>[2x]GEFMEEGKMDENEWSYHGEGNKSLVVAHAQRCVVLRFLKFPPNKKKTSEEILQHLQNIVDFGKNVMKDFLGENYVHCGEVVQLPLEFVKQLCLKIQCERPESRCDKDLDTFSGYAMCLPNLTRLQTFHFAEHRPILCVEIKPKCGFIPFSNDVTHEMKHKVCRYCMHQHLKVATGKWKKISKYCPLDLYSGNKQRMHFALRSLLQETQNNLRIFKNGE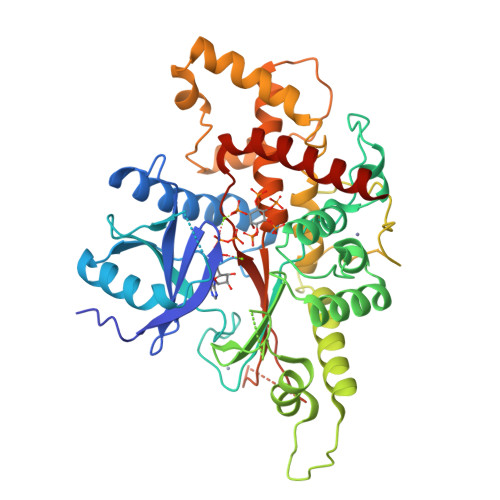LIYGCGDARSPVADLKELAHHLKPFFFPSNGLASGPHCTKAVIRELVHVITRVLLSSSEKARAGALRLGLQGPRVCEASPFSRSLHNQGKNTSEHSGLPKGCLLYKTLQVQMLDQLDIEGLYPLYKRVEQYLEEFPEERKTLQIDGPYDEVFYQKLLDLSTEDDGTVAFALTKVQQYRVAMTAKDCSIMIALSPCLQGTSSDQRPVIPSSRSRLAFSVSVLDLDLKPYESIPHQYKLDSKIVNYYSKTVHAKD> MLEQPYLDLAKKVLDEGHFKPDRTHTGTYSIFGHQMRFDLSKGFPLLTTKKVPFGLIKSELLWFLHGDTNIRFLLQHRNHIWDEWAFEKWVKSDEYHGPDMTDFGHRSQKDPEFAAVYHEEMAKFDDRVLHDDAFAAKYGDLGLVYGSQWRAWHTSKGDTIDQLGD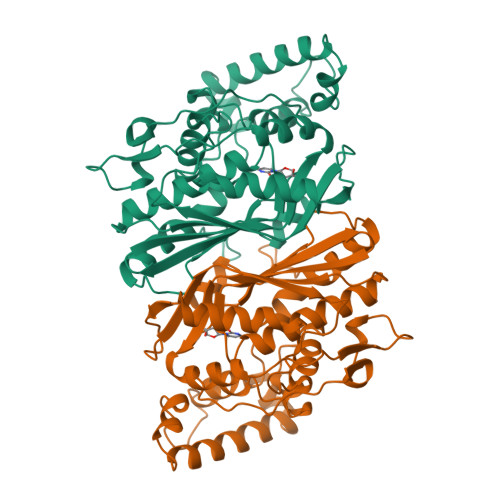VIEQIKTHPYSRKLIVSAWNPEDVPTMALPPCHTLYQFYVNDGKLSLQLYQRSADIFLGVPFNIASYALLTHLVAHECGLEVGEFIHTFGDAHLYVNHLDQIKEQLSRTPRPAPTLQLNPDKHDIFDFDMKDIKLLNYDPYPAIKAPVAV> SGSGLKELLKELNKAIASGDTETVRRILEELLELLKEAF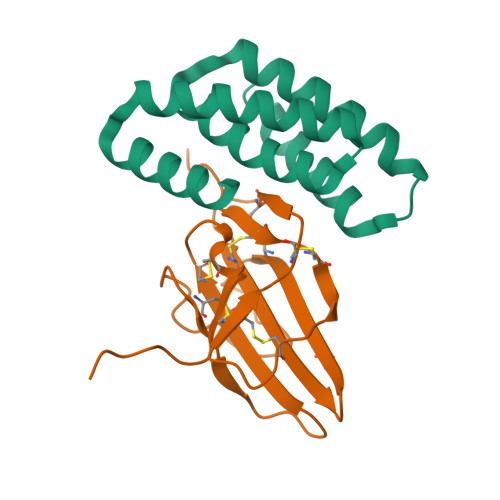EKGDYDLAISIASMAVKAASYIGDTETLKELLEILKKIKEKLKKEGDEAALKAVERNIKVVEKVA;> MKFPQLCKFCDVRFSTCDNQKSCMSNCSITSICEKPQEVCVAVWRKNDENITLETVCHDPKLPYHDFILEDAASPKCIMKEKKKPGETFFMCSCSSDECNDNIIFSEEYNT> TITVSTPIKQIFPDDAFAETIKANLKKKSVTDAVTQNELNSIDQIIANNSDIKSVQGIQYLPNVRYLALGGNKLHDISALKELTNLGWLNLSNNQLETLPQGVFEKLTNLTTLNLSNNQLTSLPQGVFERLASLTTLNLSNNNLANLNDRVFEGLTNLTTLNLSNNNLARLWKHANPGGPIYFLKGLTNLTTLNLSNNGFDELPKEVFKDLTSLTTLNLSNNQLTSLPQGVFERLTNLTTLNLSNNQLTSLPQGVFERLTNLTTLNLSNNQLTSLPQGVFERLTSLTTLNLSNNQLTSLPKGVLERLTNLKTLNLSNN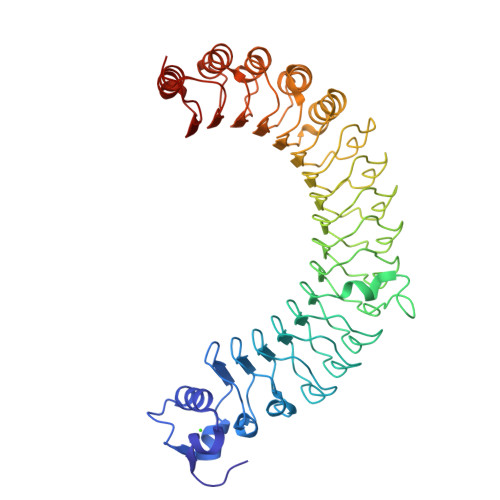QITKEVCRHVAELLKQAASLHELHLSNNNIGEEGAAELVEALLHPGSTLETLDLSNCNLTKEACREIARALKQATTLHELHLSNNNIGEEGAAELVEALLHPGSTLETLDLSNCNLTKEACREIARALKQATSLHELHLSNNNIGS> QIQPKPGFCVKTNSSEGKVFINICHSPSIPPPADVTEDELLQMLEEDQAGFRIPMSLGEPHAELDAKGQGCTAYDVAVNSNFYLRMQNSDFLRELVVTIAREGLEDKYGLQLNPEWRMLKYRSFLGSISQQNI

The R2TP complex is found in organisms from yeast to humans, and consists of the AAA+ ATPases Rvb1 and Rvb2 (human: RUVBL1 and RUVBL2), a TPR-containing protein, Tah1 (human: Spagh or RPAP3), and Pih1 (also known as NOP17 and Pih1D1, but referred to as Pih1 henceforth; Kakihara and Houry, 2012; Te et al., 2007). Pih1 is the multipoint scaffold of the R2TP complex, coupling the Rvb1-Rvb2 hetero-dodecamer, the Hsp90 chaperone machinery (via Tah1 in yeast or Spagh/RPAP3 in metazoa), and the TTT (Tel2-Tti1-Tti2) complex implicated in activation and stabilization of PIKKs (Hurov et al., 2010; Kakihara and Houry, 2012). The biological roles ascribed to the R2TP complex are directly associated with its ability to interact with the Hsp90 chaperone system and function as an Hsp90 cochaperone (Boulon et al., 2010; Izumi et al., 2012; Takai et al., 2010). Here we present crystal structures of Hsp90-Tah1-Pih1, Hsp90-Spagh/RPAP3, and Pih1-Tel2 complexes that together define key structural links within the R2TP core in yeast and in animals and reveal how R2TP connects the Hsp90 chaperone system to the TTT complex involved in PIKK activation.

Interaction with Tel2 involves the N-terminal segment of Pih1 (Horejsí et al., 2010), which contains a conserved region of unknown structure (henceforth, PIH domain). We determined the crystal structure of the mouse PIH domain1–200 with single-wavelength anomalous dispersion phasing of Tel2-peptide cocrystals (see below) grown with SeMet protein (see Experimental Procedures) and used this to phase the mPih47–179 apo and SELDpSDDEF peptide-bound structures, which were refined to 2.1 and 3.3 Å, respectively. The PIH domain consists of a twisted five-stranded β sheet with one face traversed by a helix-turn-helix segment connecting strands 4 and 5, and the other face traversed by a coil segment extending from the end of β strand 5. An additional α helix connecting strands 2 and 3 projects from the end of the sheet and packs against the larger of the other two helices. The phosphopeptide binds to an intensely basic patch in the high-resolution apo-structure formed by the loop connecting β strands 3 and 4; the faces of β strands 1, 2, and 5; and the coil segment C-terminal to β strand 5. Our structural and mutational data characterize the PIH domain as a phosphopeptide-binding domain that appears exquisitely adapted to providing specific interactions with phosphoserines (and possibly phosphothreonines) embedded in highly acidic surrounding sequences, characteristic of CK2 phosphorylation sites.>[2x]MGSSHHHHHHSSGRENLYFQGMPKLILASTSPWRRALLEKLQ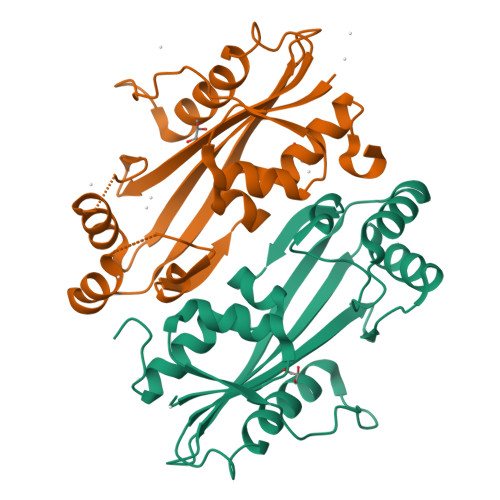ISFECAAPEVDETPRSDESPRQLVLRLAQEKAQSLASRYPDHLIIGSDQVCVLDGEITGKPLTEENARLQLRKASGNIVTFYTGLALFNSANGHLQTEVEPFDVHFRHLSEAEIDNYVRKEHPLHCAGSFKSEGFGITLFERLEGRDPNTLVGLPLIALCQMLRREGKNPLMG>[4x]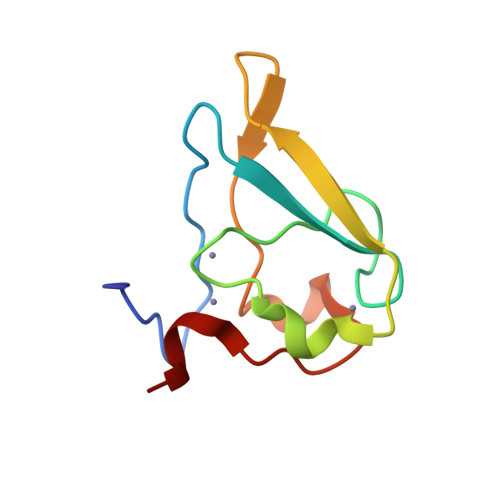GSVHKHTGRNCGRKFKIGEPLYRCHECGCDDTCVLCIHCFNPKDHVNHHVCTDICTEFTSGICDCGDEEAWNSPLHCKAEEQ;> REAA> SATNINECASNPCLNQGTCIDDVAGYKCNCLLPYTGAT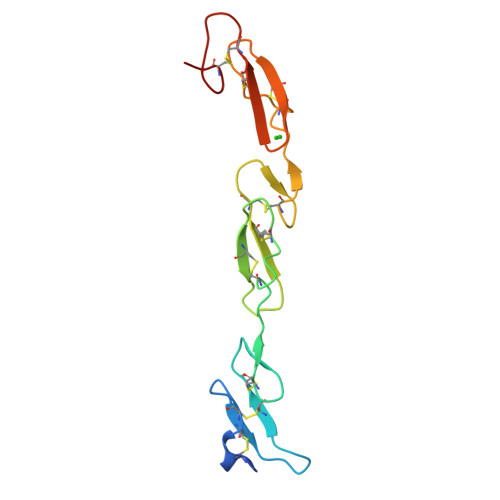CEVVLAPCAPSPCRNGGECRQSEDYESFSCVCPTGWQGQTCEVDINECVLSPCRHGASCQNTHGGYRCHCQAGYSGRNCET>[4x]ARKCSLTGKWTNDLGSNMTIGAVNSRGEFTGTYTTAVTATSNEIKESPLHGTQNTINKRTQPTFGFTVNWKFSESTTVFTGQCFIDRNGKEVLKTMWLLRSSVNDIGDDWKATRVGINIFTRLRTQKE

Egg-white avidin, similarly to streptavidin from the bacterium Streptomyces avidinii, is a small, tetrameric protein which belongs to the calycin superfamily. The interaction between avidin and biotin, its natural ligand, is one of the strongest non-covalent interactions known in biology (dissociation constant of ~10−15 M) and has been extensively characterized for more than three decades. The structural motif of this protein consists of an eight-stranded antiparallel β-barrel surrounded by flexible loops. In the present work, we have determined the first crystal structures of the avidin complexes with two fluorescent pyrene-biotin conjugates: 1-biotinylpyrene (B9P) and 1-desthiobiotinylpyrene (D9P), which were obtained via a Friedel–Crafts acylation of pyrene with biotin or desthiobiotin, respectively.

Initial co-crystallization trials in search for diffraction quality crystals of avidin in complex with B9P failed to yield single crystals. Thus, the streak seeding method was used to obtain single crystals of the avidin/B9P complex. The crystals belong to the orthorhombic space group P212121, with the unit-cell parameters a = 57.16, b = 81.95, and c = 107.89 for avidin/B9P and a = 58.97, b = 81.52, and c = 107.78 for avidin/D9P. The final models of the avidin/B9P and avidin/D9P complexes were refined to resolutions of 2.0 Å and 2.1 Å, respectively. The B9P molecule consists of the ureido ring, tetrahydrothiophene ring, valeric acid, and the pyrene moiety, while D9P molecule includes the methyl group and methylene bridge instead of the tetrahydrothiophene ring. The binding cavity in each subunit of avidin is occupied by a single ligand molecule with the same orientation, with the ring system of biotin and desthiobiotin moieties hidden deeply inside the β-barrel, while the pyrene moiety is located at the barrel entrance. The sulfur atom from the tetrahydrothiophene ring of B9P acts as an acceptor for the hydroxyl group of Thr77, while in the case of D9P there is no equivalent interaction. The fluorescence maximum was shifted to 425 nm upon the binding of B9P to avidin. The hypsochromic shift of the fluorescence maximum upon avidin/B9P complex creation may indicate that the avidin binding loops in the area of pyrene are less polar than the bulk solvent. Interestingly, we found that the crystal of avidin/B9P complex exhibited pink fluorescence upon excitation by a strong synchrotron X-ray beam during diffraction data collection.> GSHMQRVPLSVQLKPEVSPTQDIRLWVSVEDAQMHTVTIWLTVRPDMTVASLKDMVFLDYGFPPVLQQWVIGQRLARDQETLHSHGVRQNGDSAYLYLLSARNTS;> GPLGSRQDKMREEGLQLVSMIREGEAAGACPEEIFSALQYSGTEVPLQWLRSELPYVLEMVAELAGQQDPGLGAFSCQEARR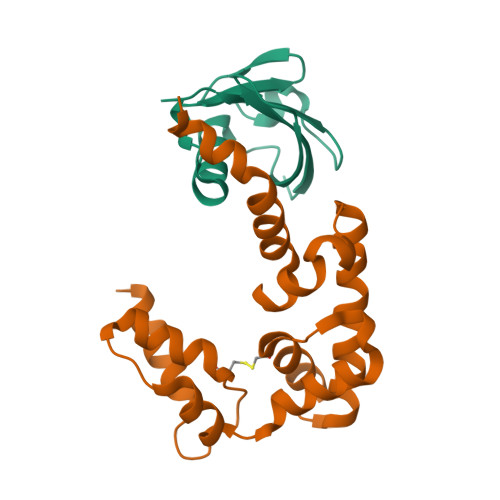AWLDRHGNLDEAVEECVRTRRRKVQELQSLGFGPEEGSLQALFQHGGDVSRALTELQRQRLEPFRQRLWDSGPEPTPSWD2-fluoranyl-5-nitro-phenol 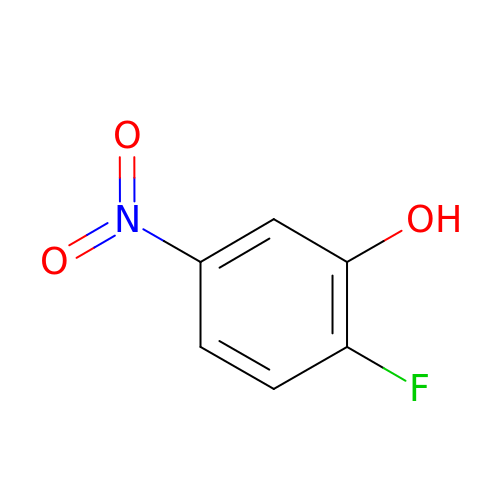| C6 H4 F N O3 | WFRLFZAMCVAQLN-UHFFFAOYSA-N(4R)-4-[3-(methylamino)-3-oxopropyl]-L-glutamic acid | C9 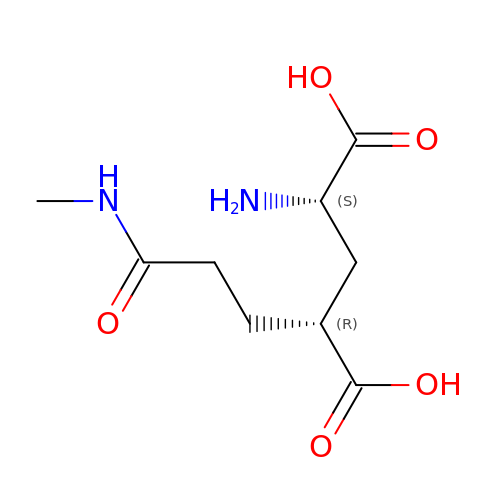H16 N2 O5 | NIJAFEMYFNBSBE-RITPCOANSA-N>[4x]AEETLMDSTTATAELGWMVHPPSGWEEVSGYDENMNTIRTYQVCNVFESSQNNWLRTKFIRRRGAHRIHVEMKFSVRDCSSIPSVPGSCKETFNLYYYEADFDLATKTFPNWMENPWVKVDTIAADESFSQVDLGGRVMKINT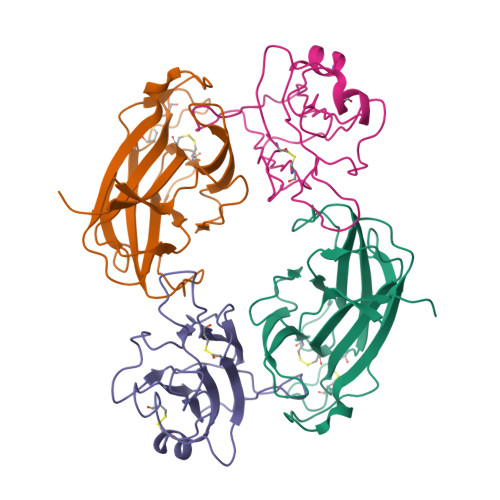EVRSFGPVSRNGFYLAFQDYGGCMSLIAVRVFYRKCPR;>[4x]IVLEPIYWNSSNSKFLPGGGLVLYPQIGDKLDIICPKVDSKTVGQYEYYKVYMVDKDQADRCTIKKENTPLLNCARPDQDVKFTIKFQEFSPNLWGLEFQKNKDYYIISTSNGSLEGLDNQEGGVCQTRAMKILMKVG>[2x]MAEAASCARKGTKYAEGTQPFTVLIEGNIGSGKTTYLNHFEKYKNDICLLTEPVEKWRNVNGVNLLELM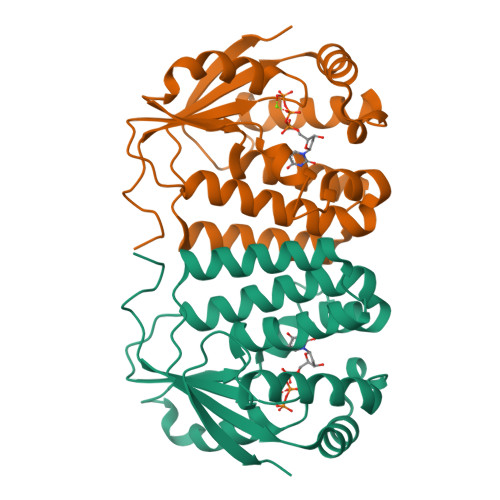YKDPKKWAMPFQSYVTLTMLQSHTAPTNKKLKIMERSIFSARYCFVENMRRNGSLEQGMYNTLEEWYKFIEESIHVQADLIIYLRTSPEVAYERIRQRARSEESCVPLKYLQELHELHEDWLIHQRRPQSCKVLVLDADLNLENIGTEYQRSESSIFDAISSNQQPSPVLVSPSKRQRVAR2-(ACETYLAMINO)-2-DEOXY-D-MANNOSE | C8 H15 N O6 | 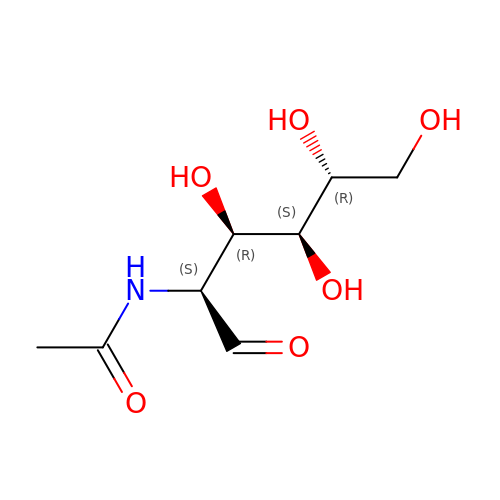MBLBDJOUHNCFQT-WCTZXXKLSA-N> MKIEEVKSTTKTQRIASHSHVKGLGLDESGLAKQAASGLVGQENAREACGVIVELIKSKKMAGRAVLLAGPPGTGKTALALAIAQELGSKVPFCPMVGSEVYSTEIKKTEVLMENFRRAIGLRIKETKEVYEGEVTELTPCETENPMGGYGKTISHVIIGLKTAKGTKQLKLDPSIFESLQKERVEAGDVIYIEANSGAVKRQGRCDTYATEFDLEAEEYVPLPKGDVHKKKEIIQDVTLHDLDVANARPQGGQDILSMMGQLMKPKKTEITDKLRGEINKVVNKYIDQGIAEL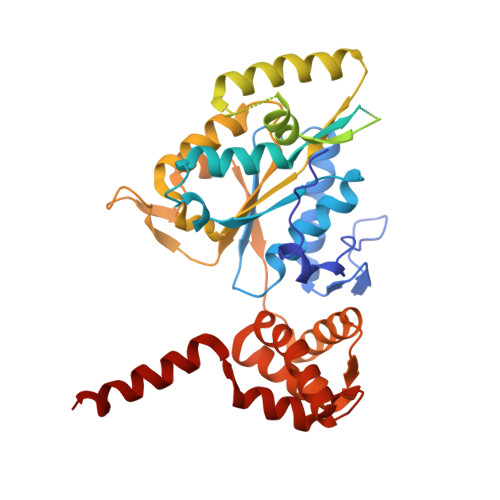VPGVLFVDEVHMLDIECFTYLHRALESSIAPIVIFASNRGNCVIRGTEDITSPHGIPLDLLDRVMIIRTMLYTPQEMKQIIKIRAQTEGINISEEALNHLGEIGTKTTLRYSVQLLTPANLLAKINGKDSIEKEHVEEISELFYDAKSSAKILADQQDKYMK Xylanases (E.C. 3.2.1.8) are hemicellulases responsible for breaking down xylan, the major hemicellulosic component of plant cell walls, into short xylooligosaccharides by a general acid–base mechanism involving two glutamic acid residues. Typically, these enzymes can be classified into glycoside hydrolase (GH) families 10 and 11 based on amino-acid sequence similarities. Recently, these enzymes have received much attention owing to their use in degradation of lignocellulosic biomass for biofuels production.

The present study reports the development of a novel endoxylanase family GH10 derived from sugarcane soil metagenome (SCXyl). Along with a comprehensive functional and biophysical characterization, three dimensional structure resolution and SAXS studies of the protein in solution, we also described the potential biotechnological application of this enzyme for biomass to bioproducts application. To the best of our knowledge, this is the first report of a three-dimensional structure for a GH10 derived from a metagenomic library. Collectively, our findings bring relevant insights on enzymatic mechanisms for production of added-value products from plant biomass.

>[2x]MSISRRLFLRNAALSAALLSIKGQAIAKAAERTGIKDFYKDDFRIGTAVATATLTMKEKKPLLALIAREFNAITPENCMKWEPLKPQDKDWHWEAADKFVEFGEKHKMYIVGHNLVWHSQVPKEVFLNESGGTISKEALTAKMQDHIATLAGRYKGRIQAWDVVNEAVEDDGSWRKSPWYNIMGEDFIAKAFTMAHEVDPKAHLIYNDYNTESPIKRNFIVGMIKNFKKQGVPIHGVGMQEHLAIDGPSVDEIEKTLIALADAGVRAHITELDIDVLPSVWNLPTAEVSTRFEYKPERDPYIQGLPKDMEEKLAKRYEDIFKIYLKHRDKIERVTLWGTADNETWLNDFPIKGRTNYPLLFDRNQKPKPAYFRLLDLKK>[2x]MDYKDDDDKGSSSSNVEVFIPVSQGNTNGFPATASNDLKAFTEGAVLSFHNICYRVKLKSGFLPCRKPVEKEILSNINGIMKPGLNAILGPTGGGKSSLLDVLAARKDPSGLSGDVLINGAPRPANFKCNSGYVVQDDVVMGTLTVRENLQFSAALRLATTMTNHEKNERINRVIQELGLDKVADSKVGTQFIRGVSGGERKRTSIGMELITDPSILFLDEPTTGLDSSTANAVLLLLKRMSKQGRT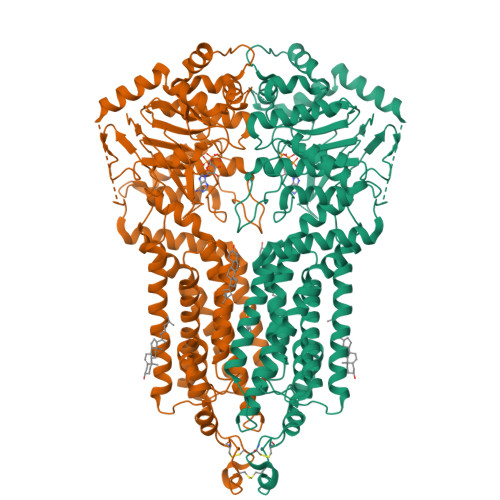IIFSIHQPRYSIFKLFDSLTLLASGRLMFHGPAQEALGYFESAGYHCEAYNNPADFFLDIINGDSTAVALNREEDFKATEIIEPSKQDKPLIEKLAEIYVNSSFYKETKAELHQLSGGEKKKKITVFKEISYTTSFCHQLRWVSKRSFKNLLGNPQASIAQIIVTVVLGLVIGAIYFGLKNDSTGIQNRAGVLFFLTTNQCFSSVSAVELFVVEKKLFIHEYISGYYRVSSYFLGKLLSDLLPMRMLPSIIFTCIVYFMLGLKPKADAFFVMMFTLMMVAYSASSMALAIAAGQSVVSVATLLMTICFVFMMIFSGLLVNLTTIASWLSWLQYFSIPRYGFTALQHNEFLGQNFCPGLNATGNNPCNYATCTGEEYLVKQGIDLSPWGLWKNHVALACMIVIFLTIAYLKLLFLKKYS>[8x]MGSSHHHHHHSSGLVPRGSSAEETIQYAAAEISASRQYTVAIETLHENLRESIADVLYMEPYEVDIDEAFIDIGMDSITGLEWIKAVNKQYGTSFTVTRVYDYPTIRDFAEMLKSELGTHLDRKIEHTDSFEAAQQKPAASSHPKPAERPLQPVQHPIKKEHEKKTVP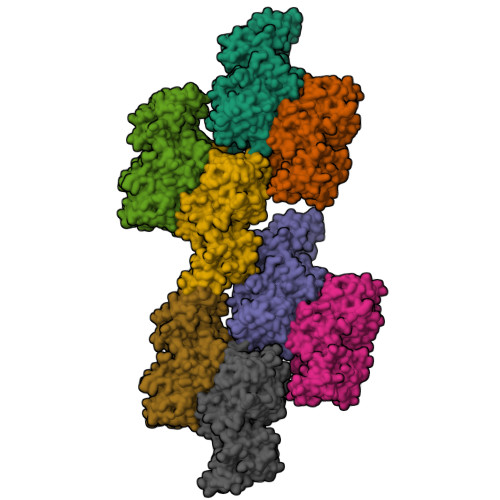VLQDRPEDAIAIVGMSGRYPGARNVREYWDNLVHARNAIRDIPTSRWDVDKYYDPVLNKKGKVYCKSMGMLDDIEHFDPLFFNIPPSEAELMDPQHRIFLQEGYKAFEDAGYNARTLNEKKCGVYLGIMSNEYGVMLNRQSRANATGNSFAIAAARIPYFLNLKGPAIPIDTACSSSLVGTHLARQALINKEIDMALVGGVSLYLTPESYMSMCEAGMLSPDGQCKAFDNGANGFVPGEGAGALVLKRLKDAEADRDHIYGIIIGSGINQDGKTNGITAPSAKSQMDLERDIYETYGIHPESISYVEMHGTGTKQGDPIELEALSTVFQEKTDKKQFCAIGSVKSNIGHTSAAAGVAGVQKVLLCMNHKTLVPTLNFTTPNEHFEFEHSPLYVNTELKPWETADGKPRRACVSSFGYSGTNAHIVIEEYQPEKRNDRLTKQHRSALFVLSAKKEKQLKAYAEAMKDFVTSNEDIDLEDMAYTLQTGREAMDYRMAFLADSREMLIKALDDYLAEMPNGSIFAAHVKTKKSEIKLFETDHDAKALLQTWIEKKRLEKVAELWVKGLQIDWNKLYGEYTPRRISLPAYPFAEEYYWLP>VQHPLDPLTKEEFLAVQTIVQNKYPISNNRLAFHYIGLDDPEKDHVLRYETHPTLVSIPRKIFVVAIINSQTHEILINLRIRSIVSDNIHNGYGFPILSVDEQSLAIKLPLKYPPFIDSVKKRGLNLSEIVCSSFTMGWFGEEKNVRTVRLDCFMKESTVNIYVRPITGITIVADLDLMKIVEYHDRDIEAVPTAENTEYQVSKQSPPFGPKQHSLTSHQPQGPGFQINGHSVSWANWKFHIGFDVRAGIVISLASIYDLEKHKSRRVLYKGYISELFVPYQDPTEEFYFKTFFDSGEFGFGLSTVSLIPNRDCPPHAQFIDTYVHSANGTPILLKNAICVFEQYGNIMWRHTENGIPNESIEESRTEVNLIVRTIVTVGNYDNVIDWEFKASGSIKPSIALSGILEIKGTNIKHKDEIKEDLHGKLVSANSIGIYHDHFYIYYLDFDIDGTHNSFEKTSLKTVRIKDGSSKRKSYWTTETQTAKTESDAKITIGLAPAELVVVNPNIKTAVGNEVGYRLIPAIPAHPLLTEDDYPQIRGAFTNYNVWVTAYNRTEKWAGGLYVDHSRGDDTLAVWTKQNREIVNK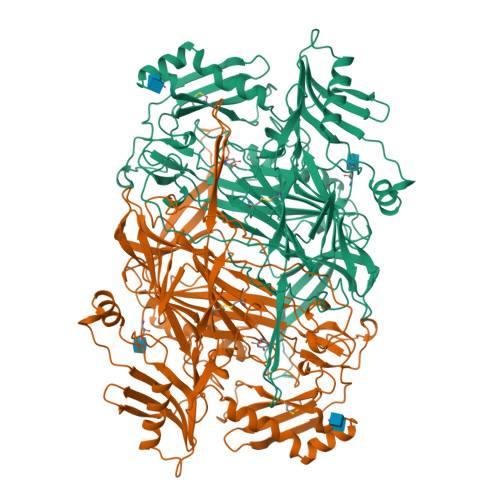DIVMWHVVGIHHVPAQEDFPIMPLLSTSFELRPTNFFERNPVLKTLSPRDVAWPGC[2x]> MELHQIRGCHKNDIELKKYNIGVAISLGNKWFSIDNIEKLVKWSLLHTKEYVIIYIADSIHGINLSVRNKLSDSHAEEVAIRYGRNLFIKIKERVSLSFSQDEQAKIIYATWSDIADSKYKEKVKYLYNLYDKNINFKNYIENFVKEWVSKEKRT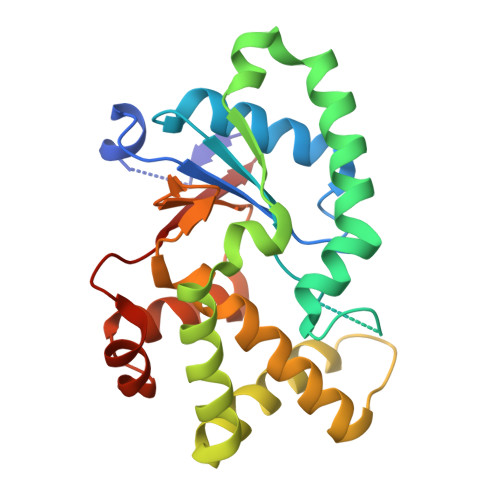FNNNEINKFGRYILEELPLLMVQVKARGVLFEAYVYPYKTRITEFVGLLQKGEIFPEIKTNILDNHPKIFLEVRE>[2x]ALETVEVMLDWYPNAVHTFLYVAIENGYFAEEGLDVDIVFPTNPTDPIQLTASGAIPLALSYQPDVILARSKDLPVVSVASVVRSPLNHVMFLAEQDFDSPADLVGLTVGYPGIPVNEPILKTMVEAAGGD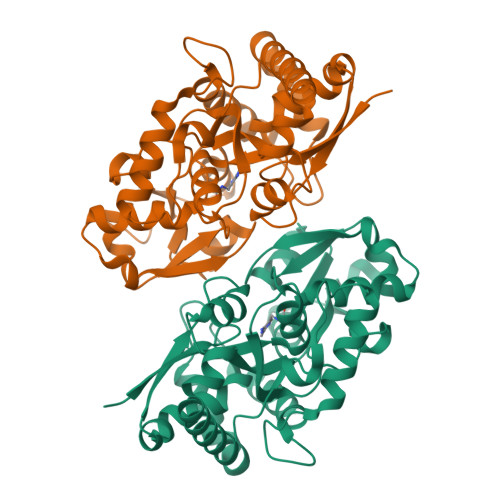YEQVHLMDVGFELGASIVSGRADAVVGTYINHEYPVLKHEGHDISYFNPVDYGVPEYDELVLISNEAYVEESGEVLAAFWRAALKGYEWMVENPDEALNVLLTNQDEANFPLIQEVEEESLSILLEKMENPNGPFGGQDAESWEEVISWLDAHDWLEQPVVAEDAFSSITD Peptidyl dipeptidase A is a highly glycosylated ectoenzyme that cleaves dipeptides from the C-terminus of a broad range of oligopeptides. AnCE is a single-domain glycosylated protein that closely shares enzymatic properties with human ACE (in particular the C-domain of human somatic ACE) and is inhibited by classic inhibitors of the human enzymes 14–17. In this study, we elucidate how the natural peptides Ang II (the principal end-product of the renin-angiotensin–aldosterone system), Arg–Pro–Pro (the BK-derived peptide) and bradykinin-potentiating peptide-b (BPPb, a snake venom inhibitor) bind to the active site of AnCE, revealing novel interactions involving several enzyme subsites. Comparison of the four structures clearly shows a common mode of peptide binding to AnCE.

Therefore, it was not surprising that the structures of AnCE in complex with BK and Thr6–BK showed Arg–Pro–Pro bound in a similar fashion in the active site cleft. Strong hydrogen bond interactions with AnCE anchor the main chain of the N-terminal Arg (P1) at the S1 site (His367, His371 and Tyr507), which is also involved in coordination with the zinc ion. Furthermore, the side chain for this residue is stabilized through contact with Tyr496. Additionally, both structures bind a citrate ion (from the crystallization medium) at the same position, making contact with the N-terminus of the bound BK (1-3) peptide. The citrate ion also interacts directly with the AnCE main chain and the surrounding water molecules. The two Pro residues at positions P1′ and P2′ form a strong interaction with AnCE through hydrogen bonds with residues His497, His337 and Tyr504, Lys495 respectively. The general mode of binding for BK (1-3) appears similar to that of Ang II, particularly through the various hydrogen bonds with AnCE. Experimental evidence suggests a preferred affinity for Pro at the S2′ binding site and highlights the importance of the hydrophobic pocket (formed by residues Phe441, Phe511, Tyr504 and Tyr507) for peptide recognition, which allows the products of BK and Thr6–BK hydrolysis to shift position and ‘register’ in the active site subsites. In both cases, complete hydrolysis of the peptide to the end point resulted in clear visible electron density for the tripeptide (Arg–Pro–Pro) in their respective crystal structures.

> ALVKEEIQAKEYLENLNKELAKRTNVETEAAWAYGSNITDENEKKKNEISAELAKFMKEVASDTTKFQWRSYQSEDLKRQFKALTKLGYAALPEDDYAELLDTLSAMESNFAKVKVCDYKDSTKCDLALDPEIEEVISKSRDHEELAYYWREFYDKAGTAVRSQFERYVELNTKAAKLNNFTSGAEAWLDEYEDDTFEQQLEDIFADIRPLYQQIHGYVRFRLRKHYGDAVVSETGPIPMHLLGNMWAQQWSEIADIVSPFPEKPLVDVSAEMEKQGYTPLKMFQMGDDFFTSMNLTKLPQDFWDKSIIEKPTDGRDLVCHASAWDFYLTDDVRIKQCTRVTQDQLFTVHHELGHIQYFLQYQHQPFVYRTGANPGFHEAVGDVLSLSVSTPKHLEKIGLLKDYVRDDEARINQLFLTALDKIVFLPFAFTMDKYRWSLFRGEVDKANWNCAFWKLRDEYSGIEPPVVRSEKDFDAPAKYHISADVEYLRYLVSFIIQFQFYKSACIKAGQYDPDNVELPLDNCDIYGSAAAGAAFHNMLSMGASKPWPDALEAFNGERIMSGKAIAEYFEPLRVWLEAENIKNNVHIGWTTSNKCVS;> RPPGFTPFR>[6x]MHHHHHHENLYFQGMSVYAIIGGTGLTQLEGLTLSESLPIETPY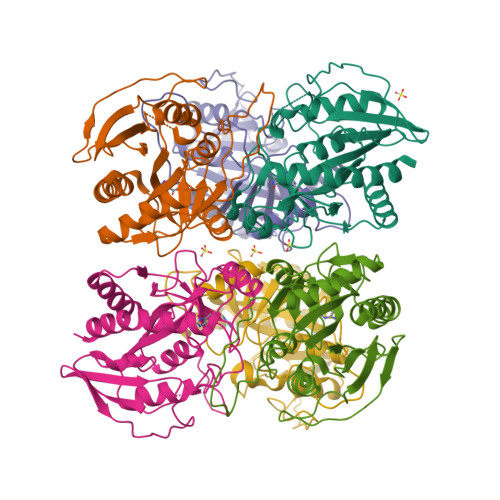GAPSAPLQRGRYAGREVLFLARHGHPHRFPPHQVNYRANLWALKQAGAEAVIAVNAVGGIHAAMGTGHLCVPHQLIDYTSGREHTYFAGDIEHVTHIDFSHPYDEPLRQRLIEALRALGLAHSSHGVYACTQGPRLETVAEIARLERDGNDIVGMTGMPEAALARELDLPYACLALVVNPAAGKSAGIITMAEIEQALHDGIGKVREVLARVLAG Human CEACAM1 (hCEACAM1) is a single pass type I transmembrane protein expressed as 12 alternatively spliced isoforms that all contain an N-terminal V set fold of the immunoglobulin superfamily (IgV) ectodomain followed by up to three type 2 constant immunoglobulin (IgC2) ectodomains (A1, B, A2), a transmembrane sequence, and a signaling cytoplasmic domain. CEACAM1 function is triggered by intercellular or trans binding of the IgV domain, resulting in higher order surface CEACAM1 oligomerization and subsequent intracellular signal transduction. In contrast to other immunoreceptors such as the T cell inhibitory and mucin domain-containing protein 3 (TIM-3), programmed cell death protein 1 (PD-1), and programmed death-ligand 1 (PD-L1), CEACAM1 serves as its own primary ligand, owing to high affinity homophilic interactions of its unique IgV domain, as well as an important microbial receptor. The displaced CC′ loop forms a cleft with the FG loop that exposes the key residues F29, S32, Y34, V39, G41, Q44, Q89, I91, N97, and E99 critical in mediating homophilic CEACAM1 interactions.

The low resolution (3.1 Å) of the I91A mutant structure limits atomic level comparison with the WT homodimer and therefore provides a more global assessment on the structural properties of the I91 residue. The I91A IgV domain adopts a GFCC′-mediated homodimer with RMSD of 0.6 Å (over 1489 atoms) compared to the WT homodimer with fewer hydrogen bonded (12 vs 17 for I99A and WT, respectively) and weaker hydrophobic interactions (specially for residue F29).

>QLTTESMPFNVAEGKEVLLLVHNLPQQLFGYSWYKGERVDGNRQIVGYAIGTQQATPGPANSGRETIYPNASLLIQNVTQNDTGFYTLQVAKSDLVNEEATGQFHVY[2x]>MANELTWHDVLAEEKQQ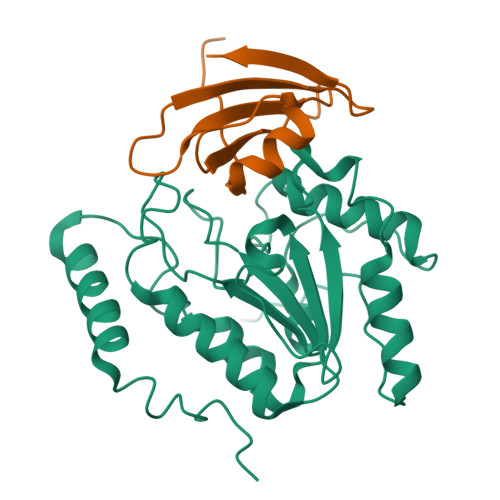PYFLNTLQTVASERQSGVTIYPPQKDVFNAFRFTELGDVKVVILGQDPYHGPGQAHGLAFSVRPGIAIPPSLLNMYKELENTIPGFTRPNHGYLESWARQGVLLLNTVLTVRAGQAHSHASLGWETFTDKVISLINQHREGVVFLLWGSHAQKKGAIIDKQRHHVLKAPHPSPLSAHRGFFGCNHFVLANQWLEQRGETPIDWMPVLPAESE[2x];>[2x]MTNLSDIIEKETGKQLVIQESILMLPEEVEEVIGNKPESDILVHTAYDESTDENVMLLTSDAPEYKPWALVIQDSNGENKIKML8-chloro-11-(1-beta-D-glucopyranuronosylpiperidin-4-ylidene)-3-hydroxy-6,11-dihydro-5H-benzo[5,6]cyclohepta[1,2-b]pyridine 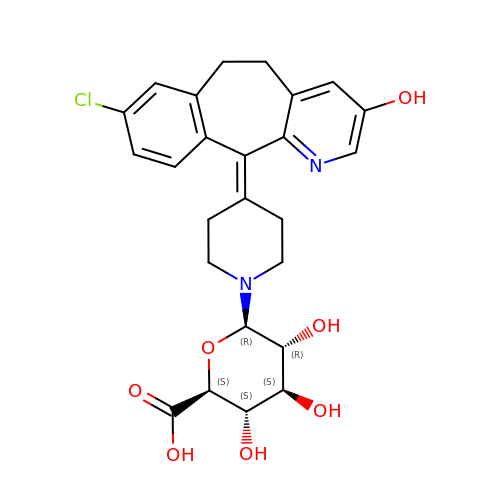| C25 H27 Cl N2 O7 | ABXRQJRQHLGUBH-OSFFKXSWSA-N>CGCGAAU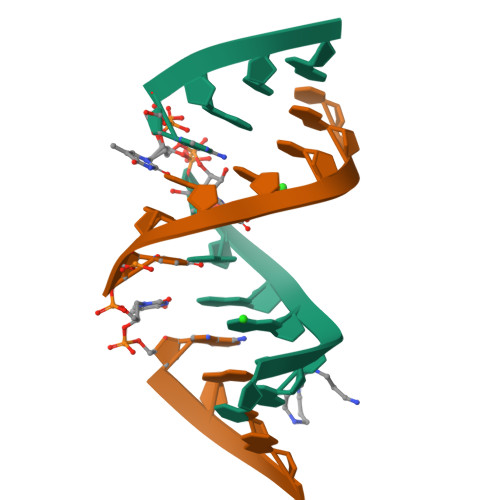XAGCG[4x]> IVGGYECKPYSQ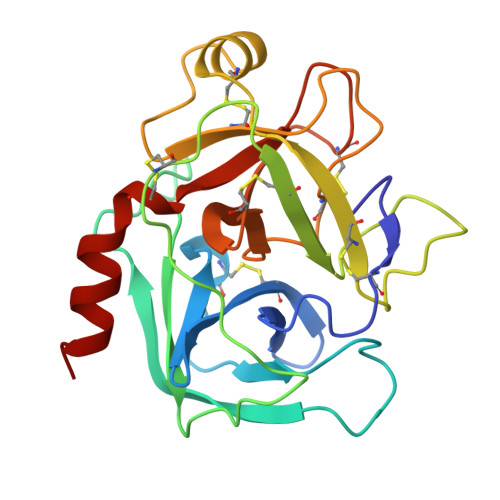PHQVSLNSGYHFCGGSLVNENWVVSAAHCYKSRVEVRLGEHNIKVTEGSEQFISSSRVIRHPNYSSYNIDNDIMLIKLSKPATLNTYVQPVALPTSCAPAGTMCTVSGWGNTMSSTADSNKLQCLNIPILSYSDCNNSYPGMITNAMFCAGYLEGGKDSCQGDSGGPVVCNGELQGVVSWGYGCAEPGNPGVYAKVCIFNDWLTSTMASY> GVVEHCCHRPCSNAEFK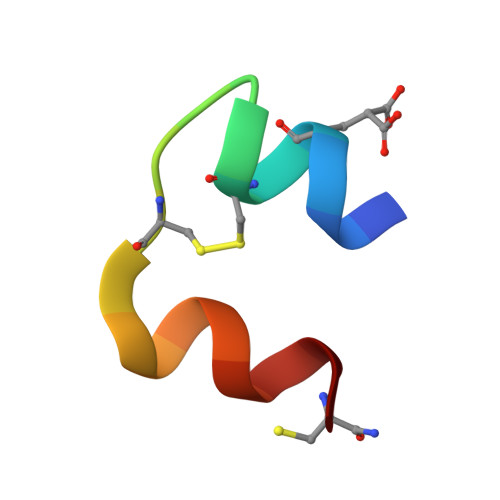KYC3-[4-(2-hydroxy-2-oxoethyl)-2,5-dimethyl-1~{H}-pyrrol-3-yl]propanoic acid | C11 H15 N O4 | 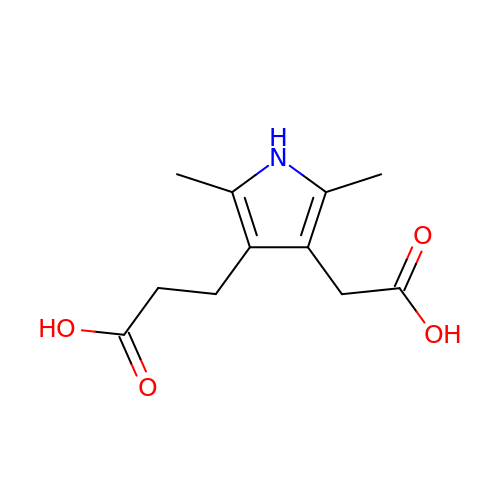KJONRYZJTCYQHI-UHFFFAOYSA-N> MLQQPTGGYTTLEQFAFTIRNDGTNATPTQFLQLLSYEATENELVKKTIPTPETHLPSARNVPGNVYIEDAITQALFGISAQNVNAHGYFSRLSALALPNTSARLGLDGVIYNSETINIPFYDPAAVANFAATYAKLGNASTPRYRADMIDIYAHVGLELAGTDAERAAGVMPVKRAKFDSWEGSLISLSRDVVNWKILAFLIDLCSLEGEALRAFKTRNRDVFRMMLFIMSTAVAANVVNRKVTKRVDRVLEYIGVNSMRTAGRTATITYDLSRHEFAAKFLQLTFTRWNAASAMIRSMPDMHTPRTSITPAGENALVRHNRYMTENFKGLSPIALA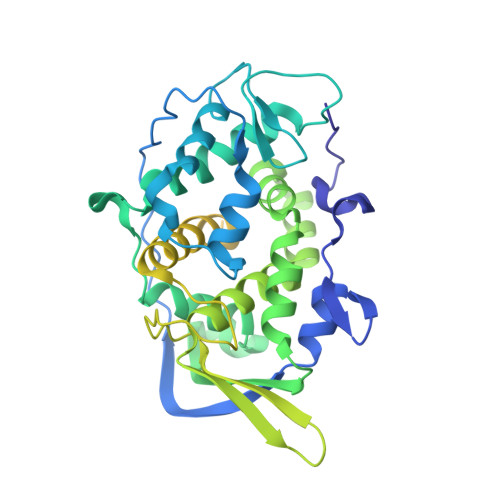QKKHEMMLHTHEIHSMDIDGSIKNMVERETVNKMNEIDAMNTAPWTEEFAEVEPTTVYERHQIGTDPEQTQLISQDAAVIVHQASSDVDENEYGNSVSELTIDTQSDSVL>MSSSEVNKVFTEEQEALVVKAWAVMKKNSAELGLQFFLKIFEIAPSAKNLFSYLKDSPVPLEQNPKLKPHATTVFVMTCESAVQLRKAGKVTVKESDLKRIGAIHFKTGVVNEHFEVTRFALLETIKEAVP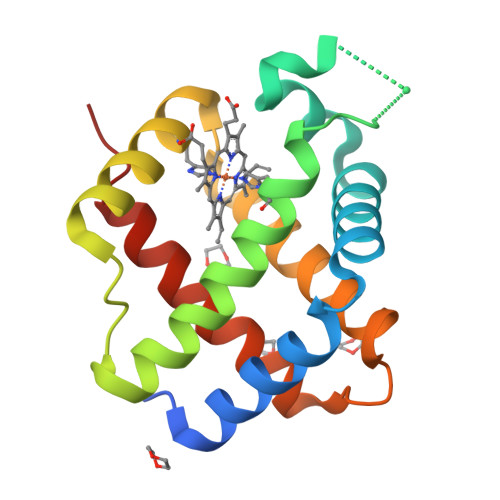EMWSPEMKNAWGVAYDQLVAAIKFEMKPSST[2x]>CCCCGGGG[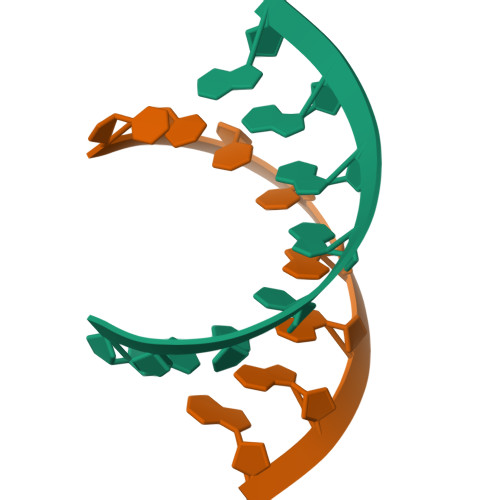2x]> MAHHHHHHSAPIADQGRAHVARSELAALDKASNGRLGVAALDTSNGTRIAHHARERFPLCGTYAVVAAAAILARASLDASLLPRRILYRRYEVVAGSPVTESHVDTGMTIAQLCAAMLQSGDKGA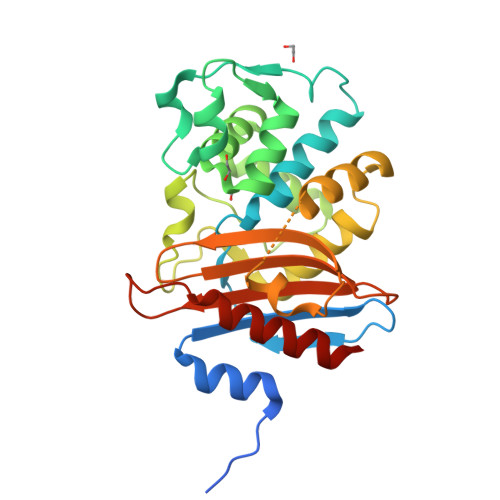GNLLMNVLGGPQAVTAFAHESGDTVFRLDRWEPELNRAAPGDERDTSTPVAMVDTLQRLLLGDTLQQAQRAQLTDWMTAGAPDATGIAAGVPPGSRVAAKRGTGGYGTTTEVAVVWPPSRAPIVLAVSFTQAQADAAARADVVASAARIATGALTATA>GMKIDGETRSARKDREIIQAATAAFISKGYDGTSMEEIATKAGASKQTVYKHFTDKETLFGEVVLSTASQVNDIIESVTTLLSEAIFMEGGLQQLARRLIAVLMDEELLKLRRLIIANADRMPQLGRAWYEKGFERMLASTASCFQKLTNRGLIQTGDPYLAASHLFG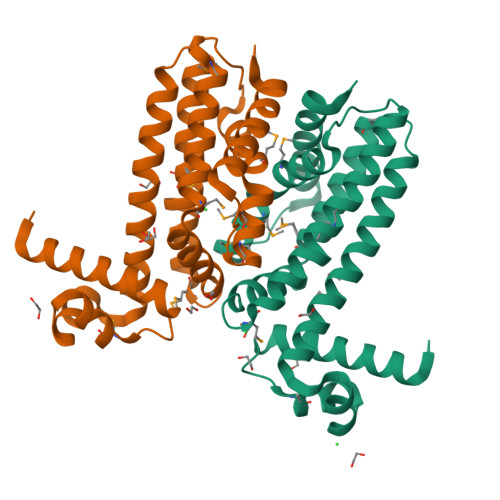MLLWIPMNEAMFTGSNRRSKAELERHADASVEAFLAVYGVQPK[2x]> GPLHMSLMDMKRTIERLVLNAKMSHDLENAKFVFVAFNYFTKALTTDVYVPAEFAACEYSLKEGIRSIYSTMIDPGQIIFGQGSDALLHSSTTHDLPLPPNALGEKNMTKLYRNIVDYLSKCQGKGKTLVVFTPAENITMVKSCFRYLESDDDFRDGGEKIQVFDIQYLLFILKKEVMNV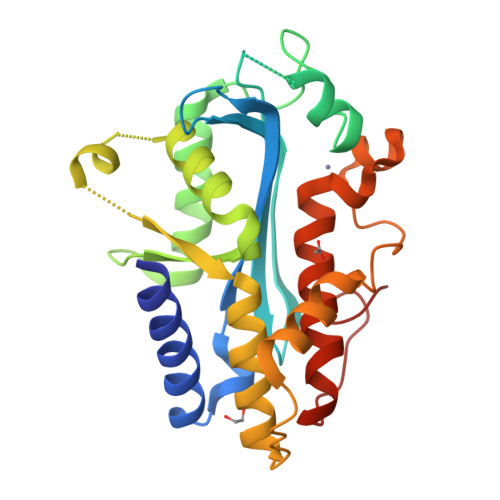ADLNDEKINKFATDAFFKKDFFEFTAGIACQYHEDNDRTKYCTQSMVTRWAYTFTDFMCGDLAITVQPGKHIPAQ Trans-methylferulate | C11 H12 O4 | 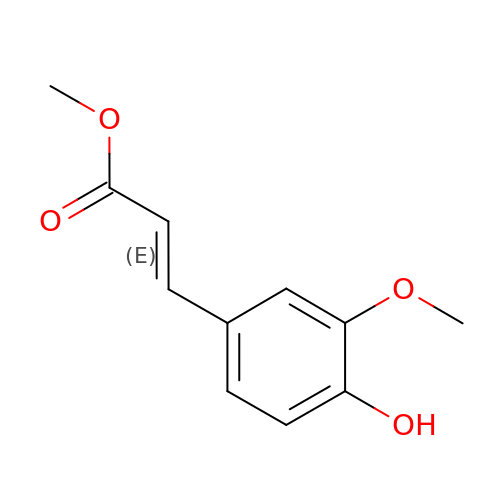AUJXJFHANFIVKH-GQCTYLIASA-N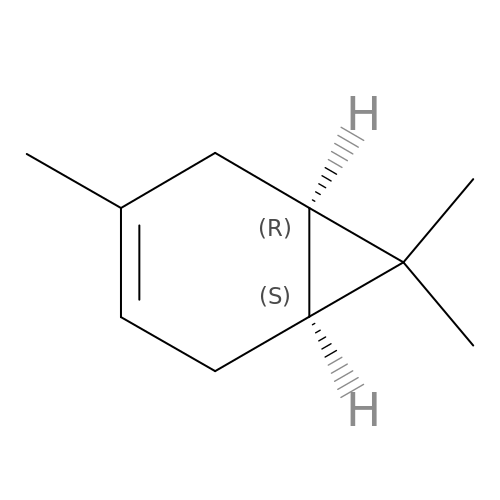(+)-3-carene | C10 H16 | BQOFWKZOCNGFEC-DTWKUNHWSA-N> AHNNEEVSGISAYLLGLIIGDGGLYKLKYKGNRSEY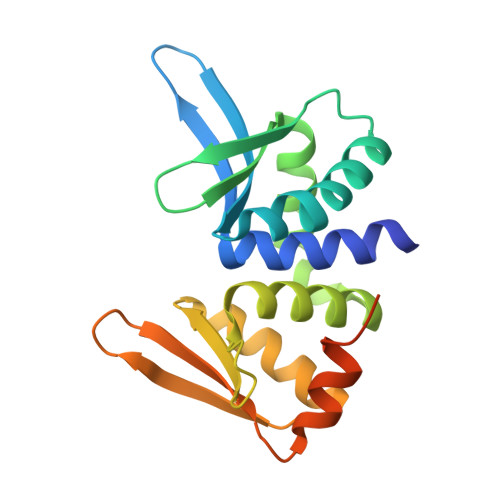RVVITQKSENLIKQHIAPLMQFLIDELNVKSKIQIVKGDTRYELRVSSKKLYYYFANMLERIRLFNMREQIAFIKGLYVAEGDKTLKRLRIWNKNKALLEIVSRWLNNLGVRNTIHLDDHRHGVYVLNISLRDRIKFVHTILSSHLNPLPPEAAALEHHHHHH> GKTITDFSISRSVLAKYE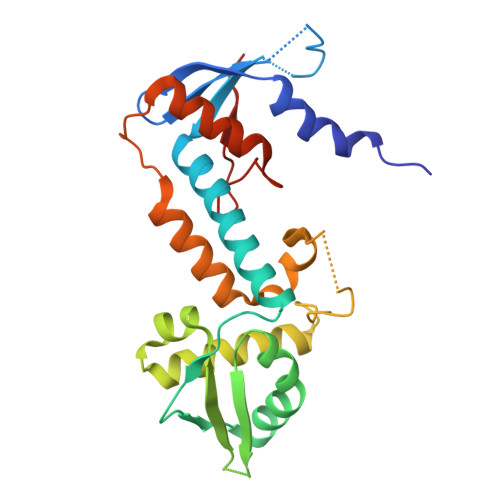VINQVDKKFILIRCLDQSIHNCPLLVLVDQHACDERIRLEELFYSLLTEVVTGTFVARDLKDCCIEVDRTEADLFKHYQSEFKKWGIGYETIEGTMETSLLEIKTLPEMLTSKYNGDKDYLKMVLLQHAHDLKDFKKLPMDLSHFENYTSVDKLYWWKYSSCVPTVFHEILNSKACRSAVMFGDELTRQECIILISKLSRCHNPFECAHGRPSMVPIAELK>LFQGPAMANSPVSVFGLGAMGTALATQFLRKGHKTTVWNRTPAKAQPLIAIGASHAPTIDSAAAASSLLIICQLDKASVMQTLQQAPTAWAAKTIVDLTNGTPAHARETADWALAHGARYIHGGIMAVPFMIGQPDAMILYSGPAEVFEGVKDTLSVLGTNTYVGEDVGLASLHDLALLSGMYGLFSGFTHAVALVQSANIPAAGFVATQLIPWLTAMTQHLNLLATQVDEKDYGDGGSSLDMQAKAAPNILEASQAQGVSVELIQPIFKLIERRVEEGKGSEGLAALVGMIMK[9x]

The NADPH-dependent imine reductase from Ajellomyces dermatitidis (AdRedAm) catalyzes the reductive amination of certain ketones with amine donors supplied in an equimolar ratio. The two AdRedAm monomers associate to form a dimer in which reciprocal domain sharing results in the formation of a large active-site cleft between the N-terminal domain of one monomer and the C-terminal domain of its partner. One of them, AdRedAm from Ajellomyces dermatitidis, has been reported to be more stable than AspRedAm and thus perhaps more suitable for process applications.

The second form, which belongs to space group C21 and was refined to 1.73 Å resolution, has nine molecules (four and a half dimers) in the asymmetric unit, each complexed with NADP+. Variations were also readily observed amongst the four dimers present in the structure from data set 2, which was obtained from crystals that grew in space group C21 and featured nine molecules in the asymmetric unit. In this structure, once again, the vast majority of backbone atoms could be modelled in subunits A–I from, in some cases, the leucine and phenylalanine residues in the purification tag at positions −5 and −4 through to Lys288. The exception was chain H, in which electron density for Gly229–Gly232 was poor and could not be modelled. In the case of data set 2, all monomers featured electron density in the omit maps that could be modelled as the cofactor NADP+. Despite the presence of the cofactor in all monomers, the difference in the conformation of some monomers was pronounced. In the most divergent examples, monomers E and I exhibited a hinge movement between the N-terminal and C-terminal domains of 14.8° as calculated using the DynDom server, with the hinge movement centred around the pendant aspartate residue Asp169. The overall effect of the hinge movement is to close the active site with respect to the cofactor, presumably to provide the hydrophobic environment that is required to favour greater stability of the transient imine intermediate.> STGSATTTPIDSLDDAYITPVQIGTPAQTLNLDFDTGSSDLWVFSSETTASEVDGQTIYTPSKSTTAKLLSGATWSISYGDGSSSSGDVYTDTVSVGGLTVTGQAVESAKKVSSSFTEDSTIDGLLGLAFSTLNTVSPTQQKTFFDNAKASLDSPVFTADLGYHAPGTYNFGFIDTTAYTGSITYTAVSTKQGFWEWTSTGYAVGSGTFKSTSIDGIADTGTTLLYLPATVVSAYWAQVSGAKSSSSVGGYVFPCSATLPSFTFGV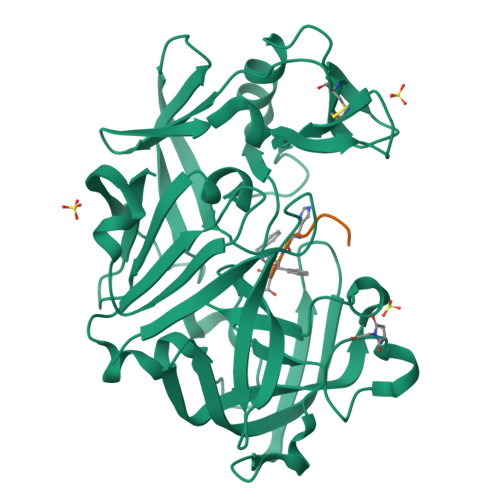GSARIVIPGDYIDFGPISTGSSSCFGGIQSSAGIGINIFGDVALKAAFVVFNGATTPTLGFASK;> HSLFHXTP>[2x]MSKSKVDNQFYSVEVGDSTFTVLKRYQNLKPIGSGAQGIVCAAYDAVLDRNVAIKKLSRPFQNQTHAKRAYRELVLMKCVNHKNIISLLNVFTPQK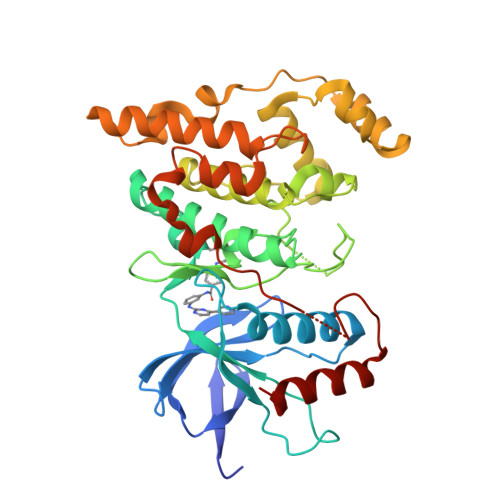TLEEFQDVYLVMELMDANLCQVIQMELDHERMSYLLYQMLCGIKHLHSAGIIHRDLKPSNIVVKSDCTLKILDFGLARTAGTSFMMTPYVVTRYYRAPEVILGMGYKENVDIWSVGCIMGEMVRHKILFPGRDYIDQWNKVIEQLGTPCPEFMKKLQPTVRNYVENRPKYAGLTFPKLFPDSLFPADSEHNKLKASQARDLLSKMLVIDPAKRISVDDALQHPYINVWYDPAEVEAPPPQIYDKQLDEREHTIEEWKELIYKEVMNSE The earlier discovery of the pathway responsible for alkane biosynthesis in cyanobacteria allowed the conversion from solar energy to alkanes through photosynthesis, without providing external carbon sources. This two-step pathway utilizes two water-soluble enzymes, namely acyl-acyl carrier protein (acyl-ACP) reductase (AAR) and aldehyde-deformylating oxygenase (ADO). AAR catalyzes the first step of this pathway, reducing the substrate fatty acyl-ACP/fatty acyl-coenzyme A (acyl-CoA) into the corresponding aldehyde in a NADPH-dependent manner. Subsequently, ADO catalyzes the conversion of fatty aldehyde into alk(a/e)ne with one carbon shorter (Cn-1 hydrocarbon) and the formate as a C1-derived form. Here we report the crystal structure of AAR from Synechococcus elongatus PCC 7942 (SeAAR) in its apo form (AARapo), together with three structures of AAR in complex with ADO from the same species of cyanobacteria (SeADO), in which AAR binds either substrate or substrate/cofactor.

In this work, we solved the AARapo structure at 2.8 Å resolution, and modeled the complete AAR protein containing 341 amino acid residues. AAR is composed of three domains: the N-terminal domain (NTD, residues 1–130), the middle domain (mid-domain, residues 131–264), and the C-terminal domain (CTD, residues 265–341). Residue C294, which is strictly conserved in AAR homologues and has been identified as the key residue for catalysis, is located approximately at the center of AAR molecule. Above C294, a wide cleft that includes the dinucleotide recognition loop is visible. In the AARapo structure, we built five molecules, which show highly similar overall architectures, in an asymmetric unit. However, three fragments, namely Fr-I (residues R19–Q29) and Fr-II (S113–T120) from the NTD, and Fr-III (V221–D235) from the mid-domain, show higher structural diversity, indicating that these regions possess an intrinsic flexibility. In fact, we found that the mobility of these fragments is pivotal for the function of AAR, as they are involved in either the interaction with ADO (Fr-I and Fr-II), or NADPH binding (Fr-III), as discussed later. In the AARapo structure, this acyl-tunnel is broken by the side chains of M279 and M21. The N-terminal segment (H7–A37) containing Fr-I is more loosely packed, potentially hindering AAR–ADO complex formation in the AARapo structure. AAR alone adopts a loose conformation as shown in the AARapo structure, which represents the resting state (ligand-free) of AAR (S0).

>MFGLIGHLTSLEQARDVSRRMGYDEYADQGLEFWSSAPPQIVDEITVTSATGKVIHGRYIESCFLPEMLAARRFKTATRKVLNAMSHAQKHGIDISALGGFTSIIFENFDLASLRQVRDTTLEFERFTTGNTHTAYVICRQVEAAAKTLGIDITQATVAVVGATGDIGSAVCRWLDLKLGVGDLILTARNQERLDNLQAELGRGKILPLEAALPEADFIVWVASMPQGVVIDPATLKQPCVLIDGGYPKNLGSKVQGEGIYVLNGGVVEHCFDIDWQIMSAAEMARPERQMFACFAEAMLLEFEGWHTNFSWGRNQITIEKMEAIGEASVRHGFQPLALAIENLYFQ[5x]> KHSLPDLPYDYGALEPHINAQIMQLHHSKHHAAYVNNLNVTEEKYQEALAKGDVTAQIALQPALKFNGGGHINHSIFWTNLSPNGGGEPKGELLEAIKRDFGSFDKFKEKLTAASVGVQGSGWGWLGFNKE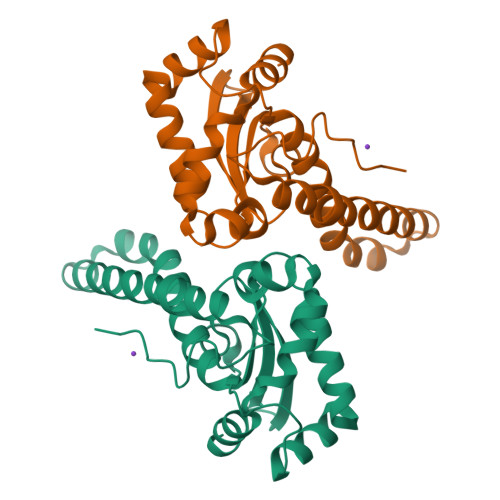RGHLQIAACPNQDPLQGTTGLIPLLGIDVWEHAYYLQYKNVRPDYLKAIWNVINWENVTERYMACKK> AEIYNKNGNKLDFYGKMVGEHVWTTNGDTSSDDTTYARIGLKGETQINDQLIGYGQWEYNMDASNVEGSQTTKTRLAFAGLKAGEYGSFDYGRNYGAIYDVEAATDMLVEWGGDGWNYTDNYMTGRTNGVATYRNSDFFGLVDGLSFALQYQGKNDHDRAIRKQNGDGFSTAATYAFDNGIALSAGYSSSNRSVDQKADG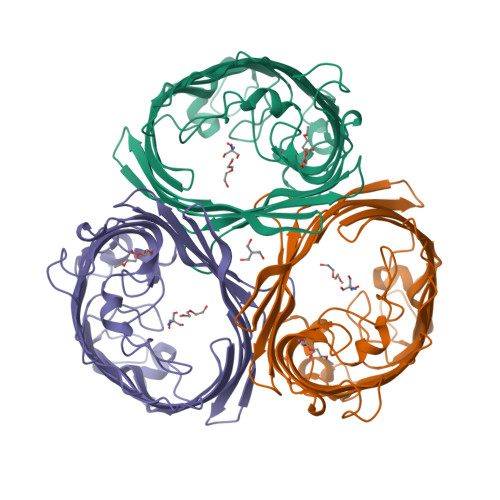NGDKAEAWATSAKYDANNIYAAVMYSQTYNMTPEEDNHFAGKTQNFEAVVQYQFDFGLRPSIGYVQTKGKDLQSRAGFSGGDADLVKYIEVGTWYYFNKNMNVYAAYKFNQLDDNDYTKAAGVATDDQAAVGIVYQF> GSGDSGSPGSVALAGNSSLCPISGWAIYSKDNGIRIGSKGDVFVIREPFISCSHLECRTFFLTQGALLNDKHSNGTVKDRSPYRTLMSCPVGEAPSPYNSRFESVAWSASACHDGISWLTIGISGPDNGAVAVLKYNGIITDTIKSWRSNILRTQESECACINGSCFTIMTDGPSNGQASYKIFKVEKGKVVKSVELNAPNYHYEECSCYPDASEVMCVCRDNWHGSNRPWVSFNQNLEYQIGYICSGVFGDNPRPNDGTGSCGPVSSNGAYGVKGFSFKYGNGVWIGRTKSTSSRSGFEMIWDPNGWTETDSSFSVKQEIVAITDWSGY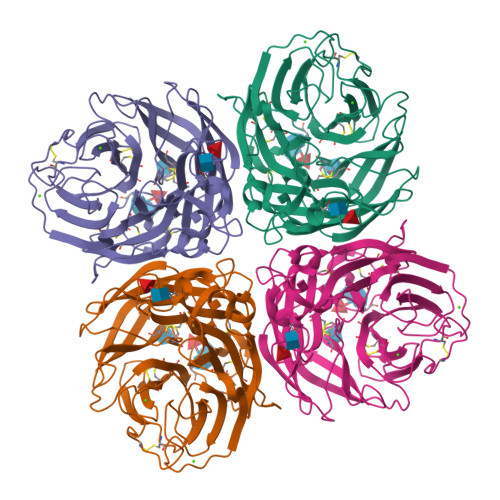SGSFVQHPELTGLDCMRPCFWVELIRGRPKENTIWTSGSSISFCGVNSDTVGWSWPDGAELPFTIDK>[2x]MTADELVFFVNGKKVVEKNADPETTLLVYLRRKLGLCGTKLGCGEGGCGACTVMISKYDRLQNKIVHFSVNACLAPICSLHHVAVTTVEGIGNTQKLHPVQERIARSHGSQCGFCTPGIVMSMYTLLRNQPEPTVEEIENAFQGNLCRCTGYRPILQGFRTFAKDGGCCGGSGNNPNCCMNQTKDQTVSLSPSLFNPEDFKPLDPTQEPIFPPELLRLKDTPQKKLRFEGERVTWIQASTMEELLDLKAQHPDAKLVVGNTEIGIEMKFKNMLFPLIVCPAWIPELNSVVHGPEGISFGASCPLSLVESVLAEEIAKLPEQKTEVFRGVMEQLRWFAGKQVKSVASIGGNIITASPISDLNPVFMASGAKLTLVSRGTRRTVRMDHTFFPGYRKTLLRPEEILLSIEIPYSKEGEFFSAFKQASRREDDIAKVTSGMRVLFKPGTIEVQELSLCFGGMADRTISALKTTPKQLSKSWNEELLQSVCAGLAEELQLAPDAPGGMVEFRRTLTLSFFFKFYLTVLQKLGRADLEDMCGKLDPTFASATLLFQKDPPANVQLFQEVPKDQSEEDMVGRPLPHLAANMQASGEAVYCDDIPRYENELSLRLVTSTRAHAKITSIDTSEAKKVPGFVCFLTAEDVPNSNATGLFN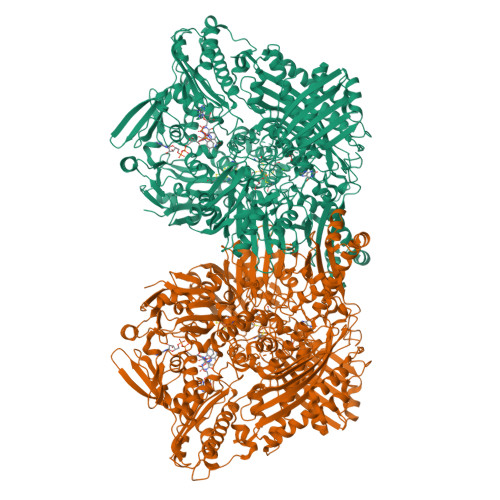DETVFAKDEVTCVGHIIGAVVADTPEHAQRAARGVKITYEDLPAIITIQDAINNNSFYGSEIKIEKGDLKKGFSEADNVVSGELYIGGQEHFYLETNCTIAVPKGEAGEMELFVSTQNTMKTQSFVAKMLGVPDNRIVVRVKRMGGGFGGKETRSTVVSTALALAAHKTGRPVRCMLDRDEDMLITGGRHPFLAKYKVGFMKTGTVVALEVAHFSNGGNTEDLSRSIMERALFHMDNAYKIPNIRGTGRICKTNLPSNTAFRGFGGPQGMLIAEYWMSEVAITCGLPAEEVRRKNMYKEGDLTHFNQKLEGFTLPRCWDECIASSQYLARKREVEKFNRENCWKKRGLCIIPTKFGISFTLPFLNQGGALVHVYTDGSVLLTHGGTEMGQGLHTKMVQVASRALKIPTSKIHISETSTNTVPNTSPTAASASADLNGQGVYEACQTILKRLEPFKKKKPTGPWEAWVMDAYTSAVSLSATGFYKTPNLGYSFETNSGNPFHYFSYGVACSEVEIDCLTGDHKNLRTDIVMDVGSSLNPAIDIGQVEGAFVQGLGLFTMEELHYSPEGSLHTRGPSTYKIPAFGSIPIEFRVSLLRDCPNKRAIYASKAVGEPPLFLASSIFFAIKDAIRAARAQHGDNAKQLFQLDSPATPEKIRNACVDQFTTL> MSTQLASNIYAPLYAPFFGFAGCAAAMVLSCLGAAIGTAKSGIGIAGIGTFKPELIMKSLIPVVMSGILAIYGLVVAVLIAGNLSPTEDYT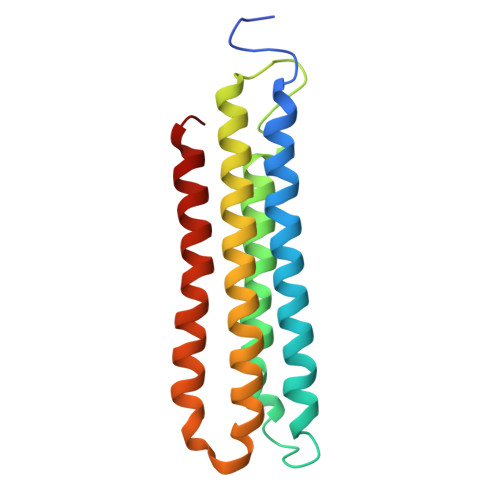LFNGFMHLSCGLCVGFACLSSGYAIGMVGDVGVRKYMHQPRLFVGIVLILIFSEVLGLYGMIVALILNTRGSE> SRANDAPIVLLHGFTGWGREEMFGFKYWGGVRGDIEQWLNDNGYRTYTLAVGPLSSNWDRACEAYAQLVGGTVDYGAAHAAKHGHARFGRTYPGLLPELKRGGRIHIIAHSQGGQTARMLVSLLENGSQEEREYAKAHNVSLSPLFEGGHHFVLSVTTIATPHDGTTLVNMVDFTDRFFDLQKAVLKAAAVASNVPYTSQVYDFK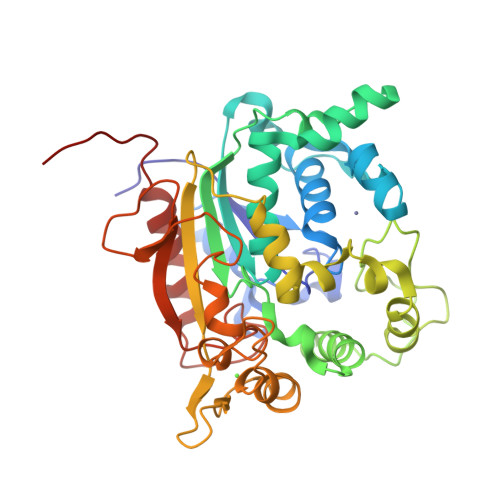LDQWGLRRQPGESFDQYFERLKRSPVWTSTDTARYDLSVPGAEKLNQWVKASPNTYYLSFTTERTYRGALTGNYYPELGMNAFSAVVCAPFLGSYRNATLGIDDRWLENDGIVNAFSMNGPKRGSTDRIVPYDGTIKKGVWNDMGTYNVDHLEVIGVDPNPLFDIRAFYLRLAEQLASLQPHHHHHH N,N'-hexane-1,4-diylbis(2,3-dihydroxybenzamide) | C20 H24 N2 O6 | 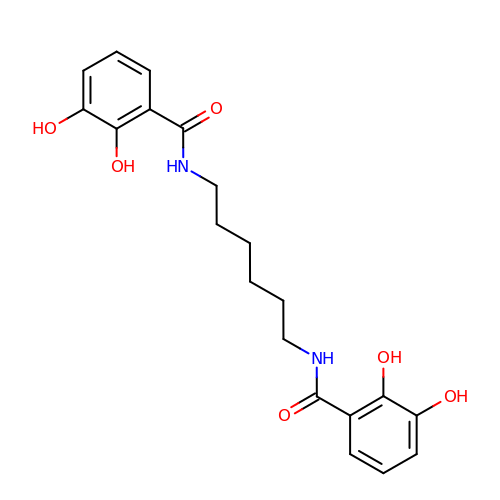JWUBPLNIABBTRS-UHFFFAOYSA-N5-fluoranyl-2-(5,6,7,8-tetrahydronaphthalen-2-ylsulfonylamino)benzoic acid | C17 H16 F N O4 S | 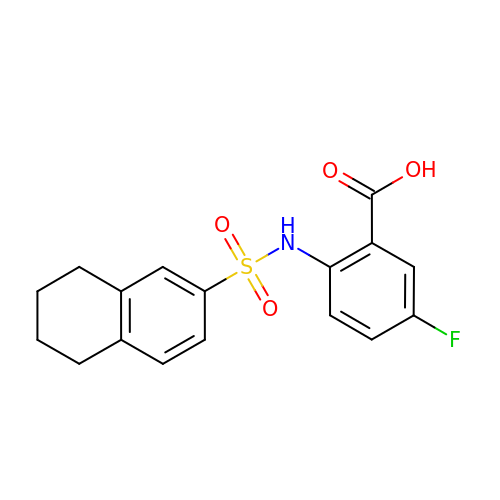AUXOWHLXYGQIFM-UHFFFAOYSA-N>STAGKVIKCKAAVLWEEKKPFSIEEVEVAPPKAHEVRIKMVATGICRTDDHVVSGTLVTPLPVIAGHEAAGIVESIGEGVTTVRPGDKVIPLFTPQCGKCRVCKHPEGNFCL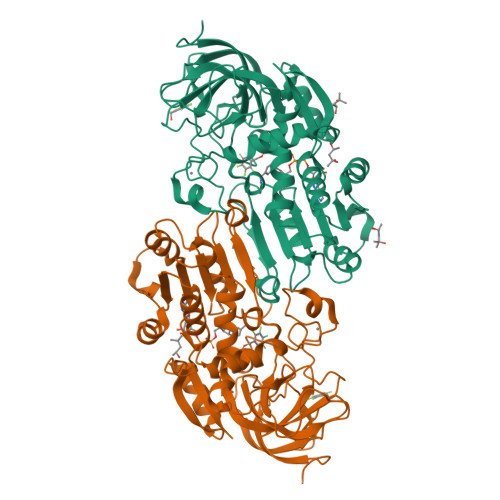KNDLSMPRGTMQDGTSRFTCRGKPIHHFLGTSTFSQYTVVDEISVAKIDAASPLEKVCLIGCGFSTGYGSAVKVAKVTQGSTCAVFGLGGVGLSVIMGCKAAGAARIIGVDINKDKFAKAKEVGATECVNPQDYKKPIQEVLTEMSNGGVDFSFEVIGRLDTMVTALSCCQEAYGVSVIVGVPPDSQNLSMNPMLLLSGRTWKGAIFGGFKSKDSVPKLVADFMAKKFALDPLITHVLPFEKINEGFDLLRSGESIRTILTF[2x]3-Deoxy-d-arabino-heptulosonate 7-phosphate synthase (DAH7PS) catalyses the first committed step of the shikimate pathway, which involves the aldol-like condensation of d-erythrose 4-phosphate (E4P) and phosphoenolpyruvate (PEP) to form 3-deoxy-d-arabino-heptulosonate 7-phosphate (DAH7P). Entry into the pathway is controlled by the allosteric regulation of DAH7PS by the pathway end products Phe, Tyr and Trp, or other intermediates of the pathway. The DAH7PS isolated from N. meningitidis (NmeDAH7PS), the causative agent of pyogenic meningitis and meningococcal septicaemia, belongs to the type Iα group. This protein adopts a homotetrameric assembly, and contains similar structural features to the other characterised type Iα DAH7PSs from Saccharomyces cerevisiae and Escherichia coli.

Of note is the single salt bridge between Arg126 and Glu27 from opposing tight dimers, which may play a role in determining the twist between tight dimers. The crystal structure of the NmeDAH7PSR126S variant was determined by X-ray diffraction. This structure was refined to a resolution of 2.0 Å and crystallised in an orthorhombic space group (P212121). Like the wild-type enzyme, the NmeDAH7PSR126S tetramer has two distinct interfaces between the chains. Superposition of the NmeDAH7PSR126S homotetramer on the NmeDAH7PSWT protein yields an RMSD of 0.61 Å (1328 Cα atoms), whereas superposition of NmeDAH7PSR126S dimeric units on those of the wild-type protein gives RMSD values between 0.18–0.25 Å. These values are consistent with the small decrease in rotation of ~2°of the dimeric units with respect to each other at the tetramer interface, and this change may also account for the difference in space group between the NmeDAH7PSR126S and NmeDAH7PSWT structures. The structural asymmetry observed in the crystal structure of NmeDAH7PSR126S may contribute to the in-solution dimerisation of this variant. Similarly, CRYSOL was used to directly compare the collected data to the hypothetical scattering from the NmeDAH7PSR126S tetramer and dimer generated from the crystal structure. These data clearly show the NmeDAH7PSR126S variant adopts a dimeric structure in solution comparable to that of the NmeDAH7PSR126S tight-dimer. The dimeric NmeDAH7PS retained its catalytic and allosteric properties.

>MTHHYPTDDIKIKEVKELLPPIAHLYELPISKEASGLVHRTRQEISDLVHGRDKRLLVIIGPCSIHDPKAALEYAERLLKLRKQYENELLIVMRVYFEKPRTTVGWKGLINDPHLDGTFDINFGLSQARSLLLSLNNMGMPASTEFLDMITPQYYADLISWGAIGARTTESQVHRELASGLSCPVGFKNGTDGNLKIAIDAIGAASHSHHFLSVTKAGHSAIVHTGGNPDCHVILRGGKEPNYDAEHVSEAAEQLRAAGVTDKLMIDCSHANSRKDYTRQMEVAQDIAAQLEQDGGNIMGVMVESHLVEGRQDKPEVYGKSITDACIGWGATEELLALLAGANKKRMARAS[4x]> MVAKGRIIRVTGPLVVADGMKGAKMYEVVRVG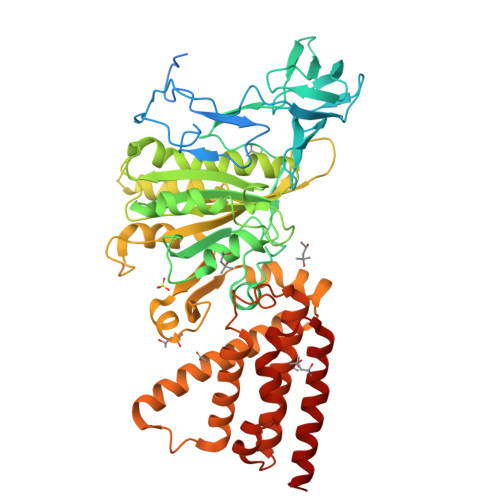ELGLIGEIIRLEGDKAVIQVYEETAGVRPGEPVVGTGASLSVELGPRLLTSIYDGIQRPLEVIREKTGDFIARGVTAPALPRDKKWHFIPKAKVGDKVVGGDIIGEVPETSIIVHKIMVPPGIEGEIVEIAEEGDYTIEEVIAKVKTPSGEIKELKMYQRWPVRVKRPYKEKLPPEVPLITGQRVIDTFFPQAKGGTAAIPGPFGSGATVTQHQLAKWSDAQVVIYIGCGERGNEMTDVLEEFPKLKDPKTGKPLMERTVLIANTSNMPVAAREASIYTGITIAEYFRDMGYDVALMADSTSRWAEALREISGRLEEMPGEEGYPAYLASKLAEFYERAGRVVTLGSDYRVGSVSVIGAVSPPGGDFSEPVVQNTLRVVKVFWALDADLARRRHFPAINWLTSYSLYVDAVKDWWHKNIDPEWKAMRDKAMALLQKESELQEIVRIVGPDALPERERAILLVARMLREDYLQQDAFDEVDTYCPPEKQVTMMRVLLNFYDKTMEAINRGVPLEEIAKLPVREEIGRMKFERDVSKIRSLIDKTNEQFEELFKKYGA>QSACTLQSETHPPLTWQKCSSGGTCTQQTGSVVIDANWRWTHATNSSTNCYDGNTWSSTLCPDNETCAKNCCLDGAAYASTYGVTTSGNSLSIGFVTQSAQKNVGARLYLMASDTTYQEFTLLGNEFSFDVDVSQLPCGLNGALYFVSMDADGGVSKYPTNTAGAKYGTGYCDSQCPRDLKFINGQANVEGWEPSSNNANTGIGGHGSCCSEMDIWEANSISEALTPHPCTTVGQEICEGDGCGGTYSDNRYGGTCDPDGCDWNPYRLGNTSFYGPGSSFTLDTTKKLTVVTQFETSGAINRYYVQNGVTFQQPNAELGS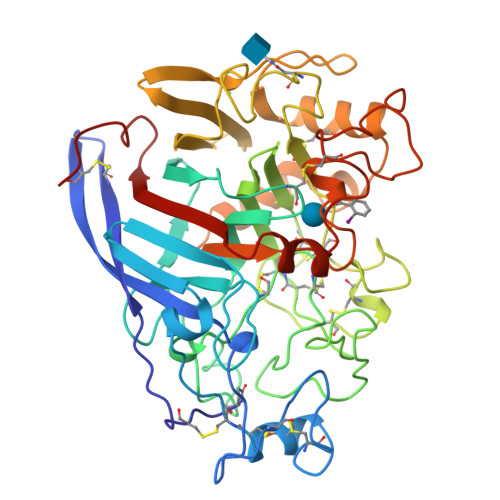YSGNELNDDYCTAEEAEFGGSSFSDKGGLTQFKKATSGGMVLVMSLWDDYYANMLWLDSTYPTNETSSTPGAVRGSCSTSSGVPAQVESQSPNAKVTFSNIKFGPIGSTGNPSG[2x]>SGLVKLGLWGGNEGTLQDIDGHPTRLTKIVIRSAHAIDALQFDYVEDGKTFAAGQWGGNGGKSDTIEFQPGEYLIAIKGTTGALGAVTNLVRSLTFISNMRTYGP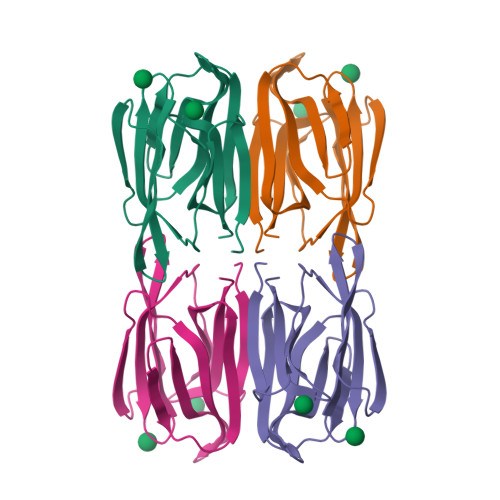FGLEHGTPFSVPVASGRIVAFYGRFGSLVDAFGIYLMPY[2x]> MACNKQNGVKNILITFTHCDTGEVIGPISHEQPDDTLPTYKTCAWTNTALTNGAVMRSASNATM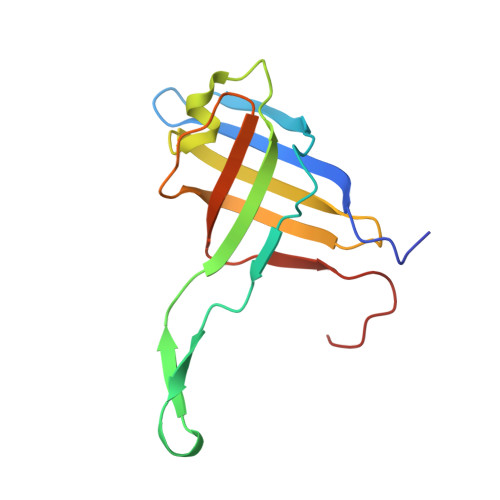TLPVVRDPRVPLAWYQGCAQIDAQVEKFDGTVMTLTEGAVTEPEESDGRAVTMTIIAAEIDELLPPGSLAAA> MRVEDVMVTDVDTIDITASLEDVLRNYVENAKGSSVVVKEGVRVGIV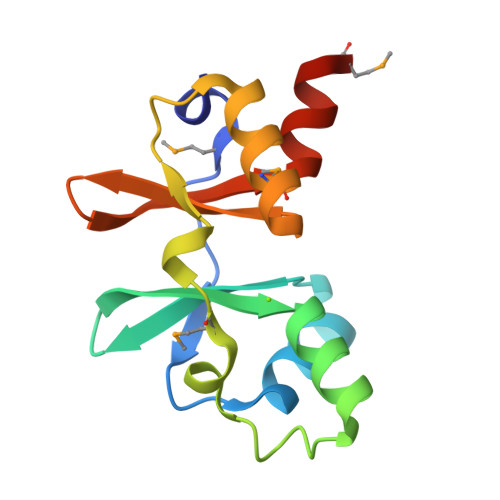TTWDVLEAIAEGDDLAEVKVWEVMERDLVTISPRATIKEAAEKMVKNVVWRLLVEEDDEIIGVISATDILRAKMAKRY>EDHPVHNLGEHSVCDSVSAWVTKTTATDIKGNTVTVMENVNLDNKVYKEYFFETKCKNPNPEPSGCRG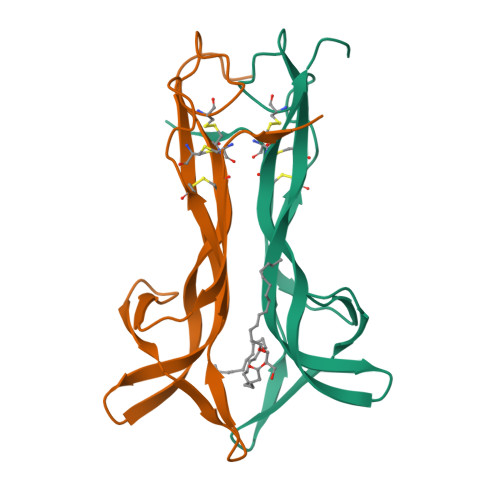IDSSHWNSYCTETDTFIKALTMEGNQASWRFIRIETACVCVITKKKGN[2x]> AQFKE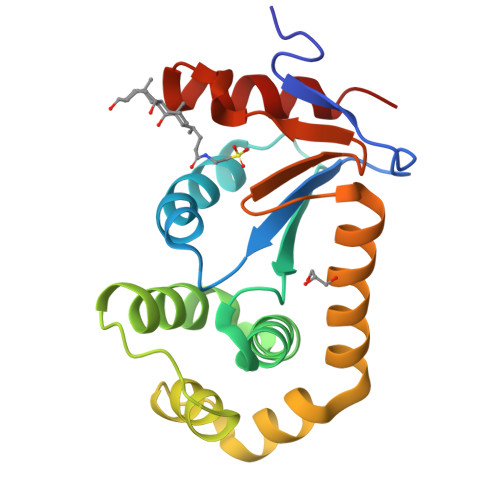GEHYQVLKTPASSSPVVSEFFSFYCPHCNTFEPIIAQLKQQLPEGAKFQKNHVSFMGGNMGQAMSKAYATMIALEVEDKMVPVMFNRIHTLRKPPKDEQELRQIFLDEGIDAAKFDAAYNGFAVDSMVRRFDKQFQDSGLTGVPAVVVNNRYLVQGQSAKSLDEYFDLVNYLLTLK>[2x]SNAMAEIKITPEELERIAGNFKN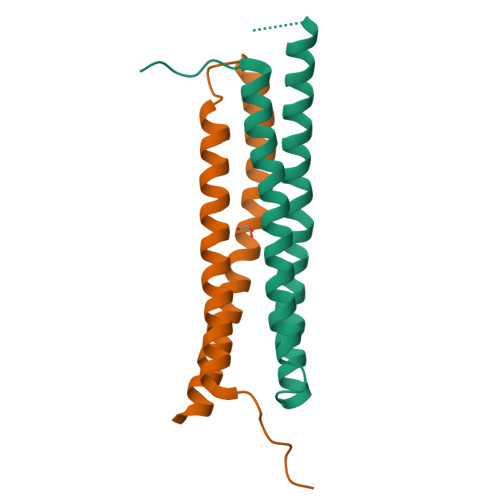AAGEAQSQINRLEGDINSLEGQWAGATQAKFRAEFIQSKQAMQQYIPILEGISTDLKRIADKFRNTDNAY> AKSNKFIIHNALSHCCLAGKVNEPQKNRILEEIEKSKANHFLILFRDSSCQFRALYTLSGETEELSRLA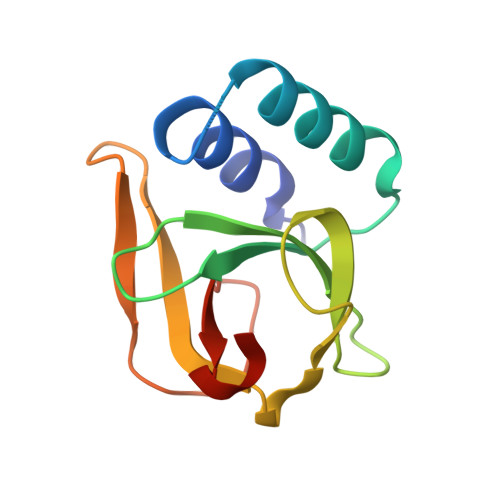GYGPRTVTPAMVEGIYKYNSDRKRFTQIPAKTMSMSVDAFTIQGHLWQSK>[6x]MAKNKIPNSRLMINYETNVDGVLKKKELPYRVLVVGDLSKGRSVDAKKEFADREVRRVNNGVDRVLEEMNISFDFEAPNFVSKDPSNLKVNYRIESVKDFRPDAVAKKVPEIRALLEMKEILASFAKDIENNRNLKKTIDMIFSDSNELESLKSKIPALTNYTIKDSCDAAESQDLSNQQVDDK;>MTINKLSLTDELLNNFGGSTEVDSVLKNIDFDVSDDASKVLSLSTDYNARNLMA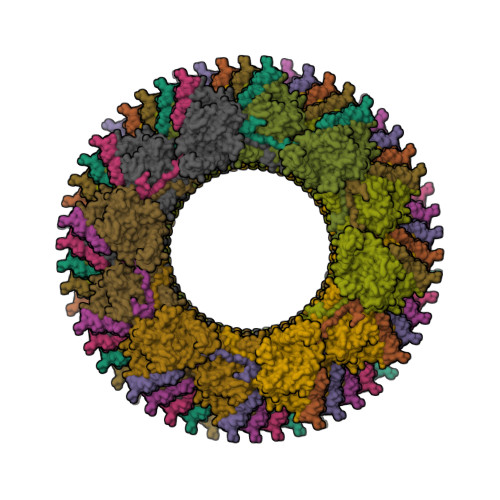LSLVLANNDNINNYNQKYIQKVITVIDKLIDLQVNSIISNDEFRALEQEWLKVQEVCQEDYDNVEVSILDVKKEELQYDFERNLYDISSSDFFKKVYVSEFDQYGGEPYGAILGLYNFENTTNDIIWLTGMGMVAKNSHAPFIASIDKSFFGVKDLSEITHIKSFEALLEHPRYKEWNDFRNLDVAAYIGLTVGDFMLRQPYNPENNPVQYKLMEGFNEFVDYDKNESYLWGPASIHLVKNMMRSYDKTRWFQYIRGVESGGYVKNLVACVYDNKGILETKSPLNVLFADYMELSLANIGLIPFVSEKGTSNACFFSVNSAKKVEEFVDGFDSANSRLIANLSYTMCISRISHYIKCVIRDKIGSIVDVESIQKILSDWISEFVTTVYQPTPLEMARYPFRNVSIEVKTIPGKPGWYSCKINVIPHIQFEGMNTTMTIDTRLEPELFGTNNN[6x]> SNAMKLALITDTSAYLPEAIENHEDVYVLDIPIIIDGKTYIEGQNLTLDQYYDKLAASKELPKTSQPSLAELDDLLCQLEKEGYTHVLGLFIAAGISGFWQNIQFLIEEHPNLTIAFPDTKITSAPQGNLVRNALMCSREGMDFDVIVNKIQSQIEKIEGFIVVNDLNHLVKGGRLSNGSAIIGNLLSIKPVLHFNEEGKIVVYEKV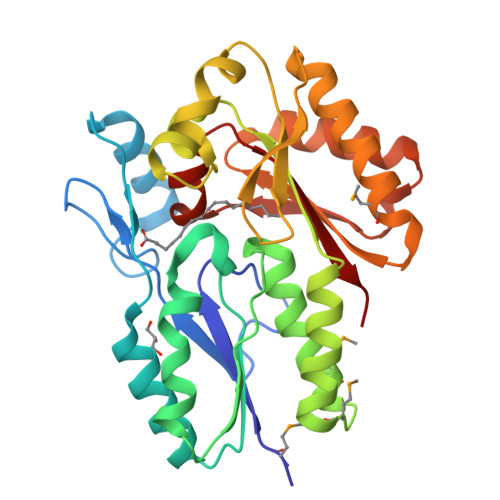RTEKKALKRLAEIVKEMTADGEYDIAIIHSRAQDKAEQLYNLLAKAGLKDDLEIVSFGGVIATHLGEGAVAFGITPKN>HHHHHHVPAFLSKLWTLVEETHTNEFITWSQNGQSFLVLDEQRFAKEILPKYFKHNNMASFVRQLNMYGFRKVVHIDSGIVKQERDGPVEFQHPYFKQGQDDLLENIKR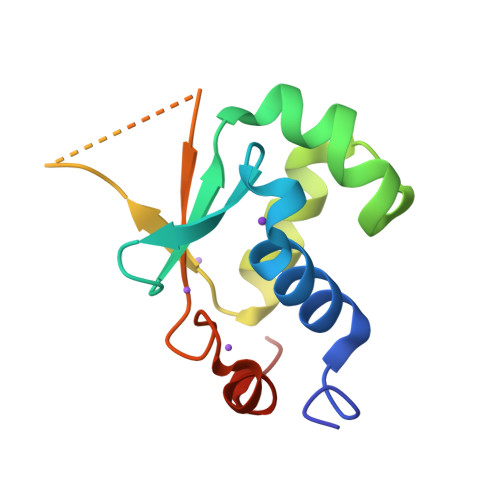KVS[4x]> 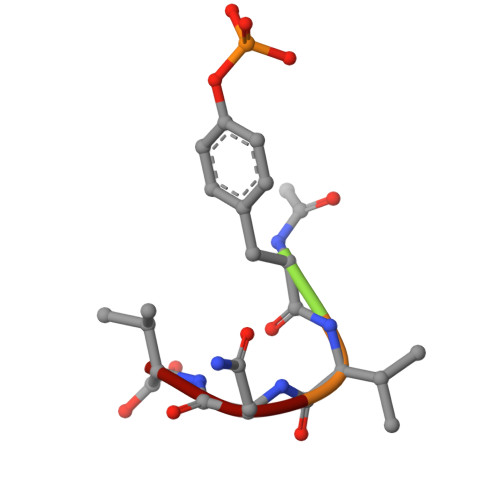XYVNV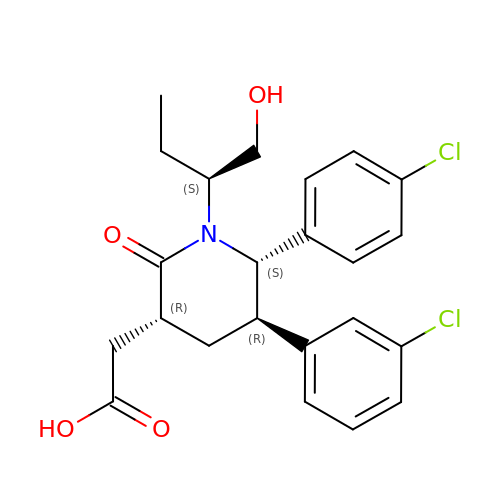{(3R,5R,6S)-5-(3-chlorophenyl)-6-(4-chlorophenyl)-1-[(2S)-1-hydroxybutan-2-yl]-2-oxopiperidin-3-yl}acetic acid | C23 H25 Cl2 N O4 | MUYVUHCWOCMQPD-CJXUKZFBSA-N>[18x]RSNVFAVDSQIPTLYMPQYISLSGVMTNDGPDNQAIASFEIRDQYITALNHLVLSLELPEVKGMGRFGYVPYVGYKCINHVSISSCNGV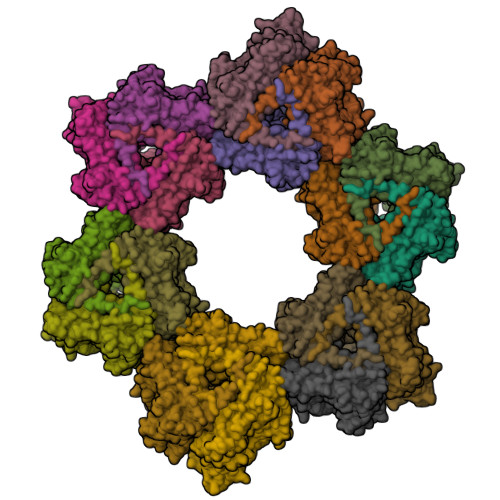IWEIEGEELYNNCINNTIALKHSGYSSELNDISIGLTPNDTIKEPSTVYVYIKTPFDVEDTFSSLKLSDSKITVTVTFNPVSDIVIRDSSFDFETFNKEFVYVPELSFIGYMVKNVQIKPSFIEKPRRVIGQINQPTATVTEVHAATSLSVYTKPYYGNTDNKFISYPGYSQDEKDYIDAYVSRLLDDLVIVSDGPPTGYPESAEIVEVPEDGIVSIQDADVYVKIDNVPDNMSVYLHTNLLMFGTRKNSFIYNISKKFSAITGTYSDATKRTIFAHISHSINIIDTSIPVSLWTSQRNVYNGDNRSAESKAKDLFINDPFIKGIDFKNKTDIISRLEVRFGNDVLYSENGPISRIYNELLTKSNNGTRTLTFNFTPKIFFRPTTITANVSRGKDKLSVRVVYSTMDVNHPIYYVQKQLVVVCNDLYKVSYDQGVSITKIMG> MRRYEVNIVLNPNLDQSQLALEKEIIQRALENYGARVEKVEELGLRRLAYPIAKDPQ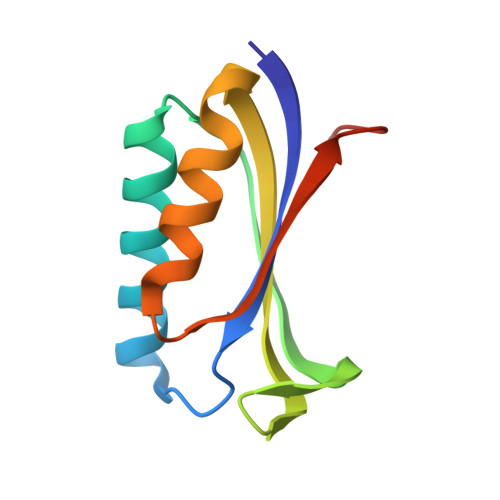GYFLWYQVEMPEDRVNDAARELRIRDNVRRVMVVKSQEPFLANA2-[(4-methyl-1H-imidazol-5-yl)methyl]-1,2,3,4-tetrahydroisoquinoline | C14 H17 N3 | 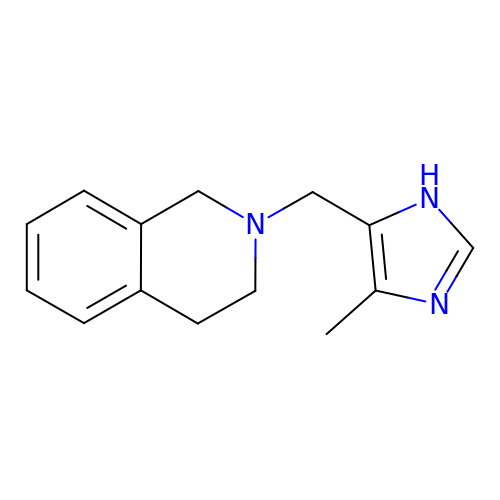YMDNLKUYUOOVMM-UHFFFAOYSA-N3,6-dichloro-2-hydroxybenzoic acid | C7 H4 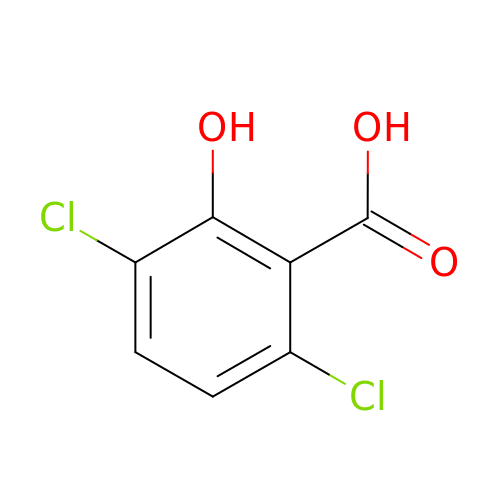Cl2 O3 | FKIKPQHMWFZFEB-UHFFFAOYSA-N ADENOSINE PHOSPHONOACETIC ACID | C12 H16 N5 O8 P | 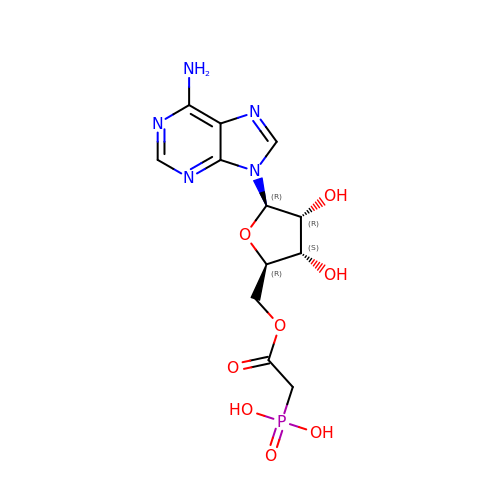KJNLSEOJEFDELT-JJNLEZRASA-N>GMSREEVESLIQEVLEVYPEKARKDRNKHLAVNDPAVTQSKKCIISNKKSQPGLMTIRGCAYAGSKGVVWGPIKDMIHISHGPVGCGQYSRAGRRNYYIGTTGVNAFVTMNFTSDFQEKDIVFGGDKKLAKLIDEVETLFPLNKGISVQSECPIGLIGDDIESVSKVKGAELSKTIVPVRCEGFRGVSQSLGHHIANDAVRDWVLGKRDEDTTFASTPYDVAIIGDYNIGGDAWSSRILLEEMGLRCVAQWSGDGSISEIELTPKVKLNLVHCYRSMNYISRHMEEKYGIPWMEYNFFGPTKTIESLRAIAAKFDESIQKKCEEVIAKYKPEWEAVVAKYRPRLEGKRVMLYIGGLRPRHVIGAYEDLGMEVVGTGYEFAHNDDYDRTMKEMGDSTLLYDDVTGYEFEEFVKRIKPDLIGSGIKEKFIFQKMGIPFREMHSWDYSGPYHGFDGFAIFARDMDMTLNNPCWKKLQAPWEASEGAEKVAASA[2x];>[2x]SQQVDKIKASYPLFLDQDYKDMLAKKRDGFEEKYPQDKIDEVFQWTTTKEYQELNFQREALTVNPAKACQPLGAVLCALGFEKTMPYVHGSQGCVAHFRSYFNRHFREPVSCVSDSMTEDAAVFGGQQNMKD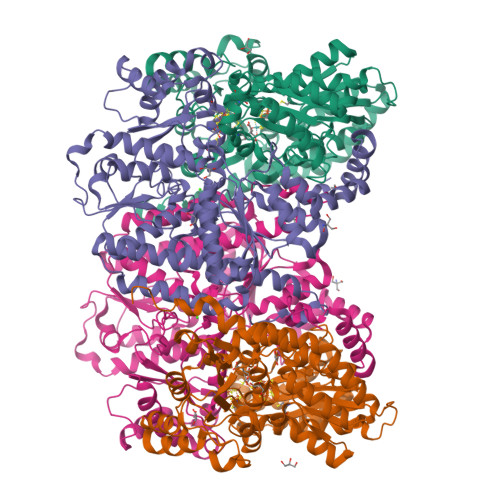GLQNCKATYKPDMIAVSTTCMAEVIGDDLNAFINNSKKEGFIPDEFPVPFAHTPSFVGSHVTGWDNMFEGIARYFTLKSMDDKVVGSNKKINIVPGFETYLGNFRVIKRMLSEMGVGYSLLSDPEEVLDTPADGQFRMYAGGTTQEEMKDAPNALNTVLLQPWHLEKTKKFVEGTWKHEVPKLNIPMGLDWTDEFLMKVSEISGQPIPASLTKERGRLVDMMTDSHTWLHGKRFALWGDPDFVMGLVKFLLELGCEPVHILCHNGNKRWKKAVDAILAASPYGKNATVYIGKDLWHLRSLVFTDKPDFMIGNSYGKFIQRDTLHKGKEFEVPLIRIGFPIFDRHHLHRSTTLGYEGAMQILTTLVNSILERLDEETRGMQATDYNHDLVR(2~{R})-~{N}-(4,5,6,7-tetrahydro-1,2-benzoxazol-3-yl)spiro[2.3]hexane-2-carboxamide | C14 H18 N2 O2 | 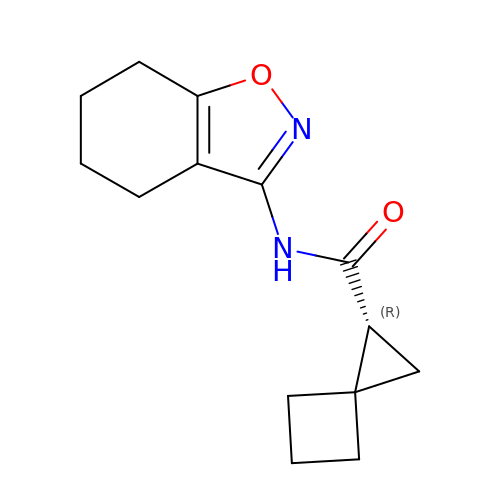LRTIDDCMWUKSQP-JTQLQIEISA-N>[2x]MSLIPLRQNIASMKGYIPGYQPPDIASWIKLNTNENPYPPSPEVVKAILEELGPDGAALRIYPSASSQKLREVAGELYGFDPSWIIMANGSDEVLNNLIRAFAAEGEEIGYVHPSYSYYGTLAEVQGARVRTFGLTGDFRIAGFPERYEGKVFFLTTPNAPLGPSFPLEYIDELARRCAGMLVLDETYAEFAE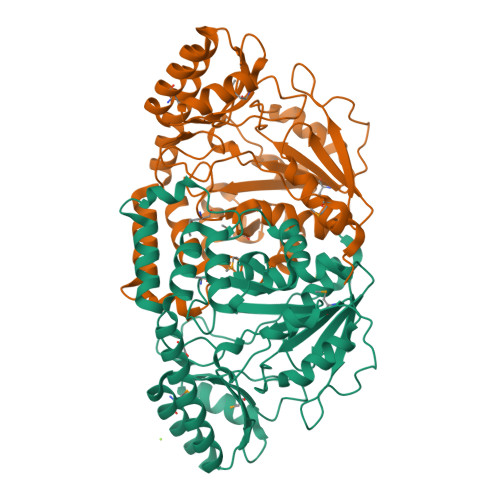SNALELVRRHENVVVTRTLSKSYSLAGMRIGLAIARPEVIAALDKIRDHYNLDRLAQAACVAALRDQAYLSECCRRIRETREWFTTELRSIGYDVIPSQGNYLFATPPDRDGKRVYDGLYARKVLVRHFSDPLLAHGMRISIGTREEMEQTLAALKEIGEGHHHHHH>MKLSGVELRRVQMPLVAPFRTSFGTASVRELLLLRAVTPAGEGWGECVTIAGPLYSSEYNDGAEHVLRHYLIPALLAAEDITAA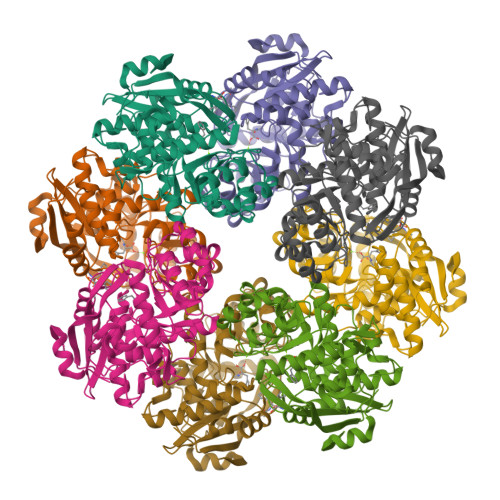KVTPLLAKFKGHRMAKGALEMAVLDAELRAHERSFAAELGSVRDSVPCGVSVGIMDTIPQLLDVVGGYLDEGYVRIKLKIEPGWDVEPVRAVRERFGDDVLLQVDANTAYTLGDAPQLARLDPFGLLLIEQPLEEEDVLGHAELARRIQTPICLDESIVSARAAADAIKLGAVQIVNIKPGRVGGYLEARRVHDVCAAHGIPVWCGDMIETGLGRAANVALASLPNFTLPGDTSASDRYYKTDITEPFVLSGGHLPVPTGPGLGVAPIPELLDEVTTAKVWIGS[4x]(2S)-2-[6-chloro-2-(4-chlorophenyl)-5-fluoro-1H-benzimidazol-1-yl]-N-cyclohexyl-2-[(2S)-oxan-2-yl]acetamide 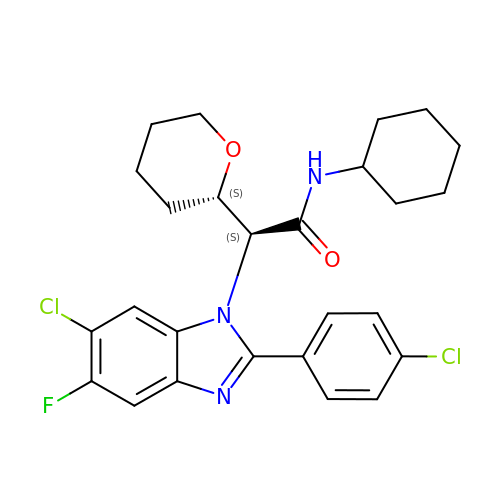| C26 H28 Cl2 F N3 O2 | GSCSJUCYZMUKCP-ZEQRLZLVSA-N> MGLLRLLVLCTLAACCMARSPPAPPLPQRPLSPLHPLGCNDSEVLAVAGFALQNINRDQKDGYMLSLNRVHDVREHY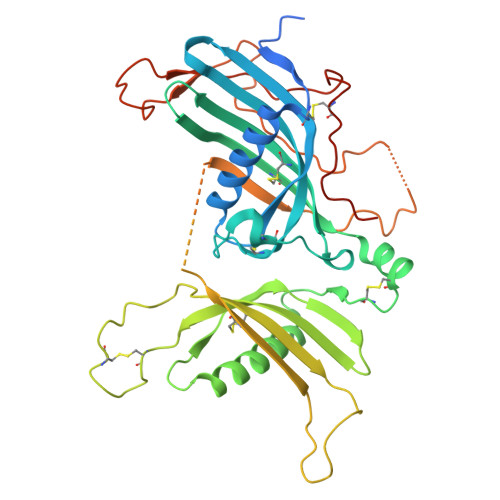QEDMGSLFYLTLDVLETDCHVLSRKAQKDCKPRMFYESVYGQCKAMFHINKPRRVLYLPAYNCTLRPVSKRKTHTTCPDCPSPIDLSNPSALEAATESLAKFNSKSPSKKYELVKVTKAMNQWVSGPAYYVEYLIKEAPCTKSQASCSLQHSDSEPVGICQGSTVQSSLRHVPLIQPVEKSVTVTCEFFESQAQVPGDENPAVTQGPQKLPQKNTAPTSSPSVTAPRGSIQHLPELDDEKPEESKGGSPEEAFPVQLDLTTNPQGDTLDVSFLYLEPGDKKLVVLPFPGKEQRSAECPGPEKENNPLVLPPHHHHHH> MTDLKASSLRALKLMDLTTLNDDDTDEKVIALCHQAKTPVGNTAAICIYPRFIPIARETLKEQGTPEIRIATVTNFPHGNDDIDIALAETRAAIAWGADEVDVVFPYRAL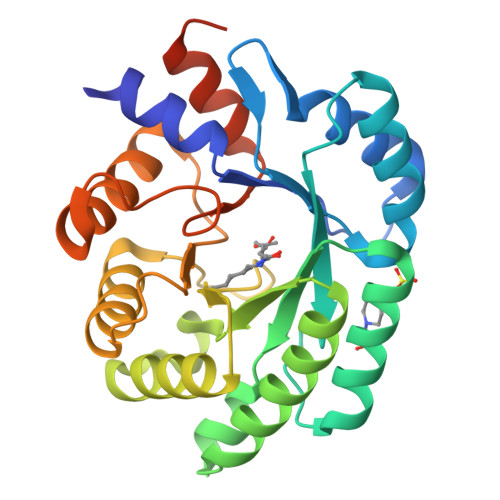MAGNEQVGFDLVKACKEACAAANVLLKVIIETGELKDEALIRKASEISIKAGADFIKTSTGKVAVNATPESARIMMEVIRDMGVEKTVGFKPAGGVRTAEDAQKYLAIADELFGADWADARHYRFGASSLLASLLKALGHGDGKSASSYHHHHHH>[2x]MGSTEYKPTVRLATRDDVPRAVRTLAAAFADYPATRHTVDPDRHIERVTELQELFLTRVGLDIGKVWVADDGAAVAVWTTPESVEAGAVFAEIGPRMAELSGSRLAAQQQMEGLLAPHRPKEPAWFLATVGVSPDHQGKGLGSAVVLPGVEAAERAGVPAFLETSAPRNLPFYERLGFTVTADVEVPEGPRTWCMTRKPGASHHHHHH

Puromycin and the Streptomyces alboniger-derived puromycin N-acetyltransferase (PAC) enzyme form a commonly used system for selecting stably transfected cultured cells. The crystal structure of PAC has been solved using X-ray crystallography, revealing it to be a member of the GCN5-related N-acetyltransferase (GNAT) family of acetyltransferases. PAC adopts a fold consistent with the GCN5-related N-acetyltransferase (GNAT) family, consisting of a seven-stranded β-sheet interspersed with four α-helices. PAC displays the typical structural hallmarks of this family which includes a cleft in the middle of the sheet between the parallel strands 4 and 5 that facilitates AcCoA binding.

The poor initial electron density around the adenine moiety of the CoA made its unambiguous placement difficult and the adenine moiety has been modelled in both orientations. In the two crystal structures obtained in this work, with either AcCoA bound, or the trapped reaction products (CoA and acetylated-puromycin) in the other, the absence of puromycin causes little change to the global structure of PAC. The entry point of the acetyl acceptor substrate puromycin is proximal to the AcCoA-binding region, and this is also where most structural differences can be observed relative to other GNAT enzymes. The most distinctive feature is the insertion of an α-helical hairpin between β-strands 3 and 4 (Fig. 1b dark-purple helices); this forms the entry point for puromycin into the active site. The electrostatic potential of the lining of the active site is polarised: it has a predominantly negative potential for the puromycin-binding site and the opposed positive potential for the AcCoA-binding site. Rather, it is likely PAC facilitates the direct acetyl group transfer through the geometric placement of the puromycin amino group to carry out a nucleophilic attack on the acetyl group of the donor. Based on our crystal structure, the general acid required to protonate the nascent CoA thiol is very likely to be Y171, which is consistent with other GNAT enzymes by its proximity to the CoA thiol. A candidate for this could be E161, but its direct engagement in puromycin binding would make it difficult to dissect which of these roles would be affected by mutation.>[2x]MAYVEIIEQPKQRGMRFRYKCEGRSAGSIPGERSTDTTKTHPTIKINGYTGPGTVRISLVTKDPPHRPHPHELVGKDCRDGYYEADLCPDRSIHSFQNLGIQCVKKRDLEQAISQRIQTNNNPFHVPIEEQRGDYDLNAVRLCFQVTVRDPAGRPLLLTPVLSHPIFDNRAPNTAELKICRVNRNSGSCLGGDEIFLLCDKVQKEDIEVYFTGPGWEARGSFSQADVHRQVAIVFRTPPYADPSLQAPVRVSMQLRRPSDRELSEPMEFQYLPD;>[2x]MGPYLQILEQPKQRGFRFRYVCEGPSHGGLPGASSEKNKKSYPQVKICNYVGPAKVIVQLVTNGKNIHLHAHSLVGKHCEDGVCTVTAGPKDM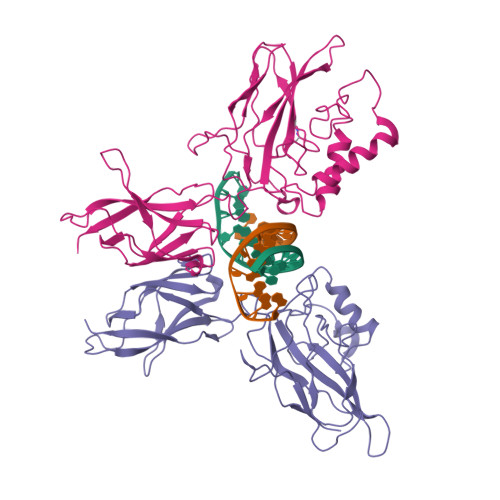VVGFANLGILHVTKKKVFETLEARMTEACIRGYNPGLLVHSDLAYLQAEGGGDRQLTDREKEIIRQAAVQQTKEMDLSVVRLMFTAFLPDSTGSFTRRLEPVVSDAIYDSKAPNASNLKIVRMDRTAGCVTGGEEIYLLCDKVQKDDIQIRFYEEEENGGVWEGFGDFSPTDVHRQFAIVFKTPKYKDVNITKPASVFVQLRRKSDLETSEPKPFLYYPE> MAKHATPLLDQLQSGPWPSFVADIKEEAERRHSNQDNVEYQIPVDVCDDLLGILELKYSDGTTHWKHGGIVGVFGYGGGVIGRYCDQPQMFPGVAHFHTVRVAQPAGMYYTTDFLKQLCDLWDMRGSGLTNMHGATGDIVLLGTTTPQLEEFYFELTHKMNNDLGGSGSNLRTPASCLGDSRCEWACYDAQELCYQMTQEYQDE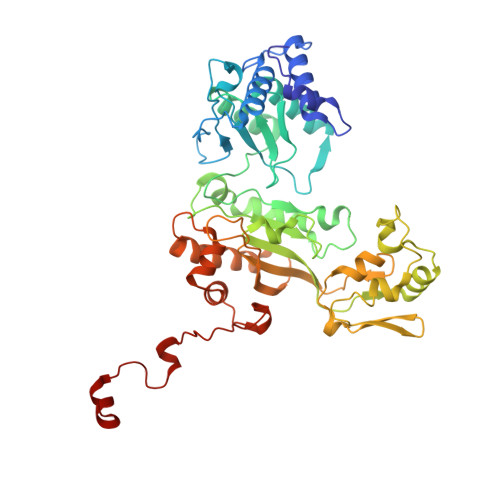LHRPAFPYKFKFKFDGCPNGCVASIARSDMSFIGTWRDDIRIDQEAVAAYVGGEIQPNGGAHSGKDWGAFDIQKEVIDLCPTECMWMEDGKLQINNRECTRCMHCLNVMPRALRIGNDRGLSILVGAKAPILDGAQMGSLLVPFIKVEDPYDEIKEIIEGIWEWWMEEGKNRERLGELIKRQGLAKAIAAVGLTPVPQHVMEPRHNPYIFWKEKDVEGGWDRDIADYRKHHQR>[4x]MASHHHHHHHENLYFQGMSGIQTVSKSATDLTEMVKKITTMNRGEFRQITLATGAGKTTELPRSVIEEIGRHKRVLVLIPLRAAAESVYQYMRQKHPSIAFNLRIGEMKEGDMATGITYASYGYFCQMSQPKLRAAMVEYSFIFLDEYHCATPEQLAIMGKIHRFSENLRVVAMTATPA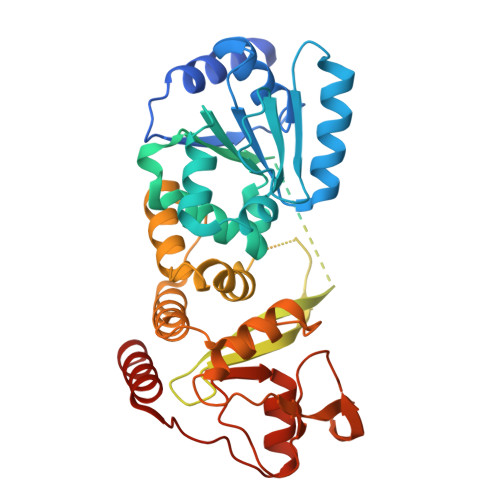GTVTTTGQKHPIEEFIAPEVMKGEDLGSEYLDIAGLKIPVEEMKNNMLVFVPTRNMAVEAAKKLKAKGYNSGYYYSGEDPSNLRVVTSQSPYVVVATNAIESGVTLPDLDVVVDTGLKCEKRIRLSPKMPFIVTGLKRMAVTIGEQAQRRGRVGRVKPGRYYRSQETPVGSKDYHYDLLQAQRYGIEDGINITKSFREMNYDWSLYEEDSLMITQLEILNNLLISEELPMAVKNIMARTDHPEPIQLAYNSYETQVPVLFPKIRNGEVTDTYDNYTFLNARKLGDDVPPYVYATEDEDLAVELLGLDWPDPGNQGTVEAGRALKQVVGLSTAENALL> MEIALERIYGHRLALPQVGAALLFAQEAPPALLLVPEARLRRYRDLSAFGAKVYVNPGLEALEEKALFVLSYEEALSPFPEDPEAWRLLLEVGRAYPREALLSRLLKLGYARDEDYRVLGEVVELGEVRLEFFGDELERLVVRGEERRRHVLLPKPGKAEGFTSKKVLHFPGPVYLDTPALAPKALWPLLAGRPWVALGGGVELPPLELGARPLPPYRGSLKALEKDLARWLAEGKRVHLFVGHARTLEYLKRRLQAFSPLILDRFPGPKGRLALLPGDFEGGAEWGEWVLLTEALVFATGGVRARVRVGEGLSDPGALSPGDYLIHPEHGVGQYLGLETREVLGVKRDYLVLRYKGEGKLYLPVEQLPLLKRHPGTTDDPPELSSLGKNEWQRAKEKARKDVEELAGRLLVLQAKRKATPGRAFPPLPEWDPLVEKGFPYELTPDQKRALEEVLRDLESPHPMDRLVSGDVGFGKTEVALRAAHRVVGHGAQVAFLVPTTLLAEQHGKTFRERFQGLPVRVAVLSRFTPPKEEEAILKGLAEGTVDIVIGTHRLLQEDVRFRDLGLLIVDEEHRFGVAQKERIRELKAEVDTLYLSATPIPRTLYSALVGLKDLSSIQTPPPGRKPIKTFLAPFDPLLVREAILFELERGGKVFYVHDRVASIEARRRFLESLVPEARIGVVHGQMPESLIEETMLLFAEGAYDVLLATTIIEAGLDVPEANTILIERADRLGLATLYQLRGRVGRREEEAYAYLFHPPRLTEAAEKRLAAIADLSDLGSGHLLAERDMEIRGVGNLLGPEQHGHIRALSLEVYTELLEEAIRKLKGEVKEERRHVTLDLALSARLPAEYVGSLEARSRYYSRFAEAKSLAELSRLVRELKERYGPLPEEAENFVALARLRLVAERKGVVSITEGLTHLEVVFPRYPLDYDARGLKGLPYRVELTQYPPGFRLEKKGLRPRDYPEALMEVLYLF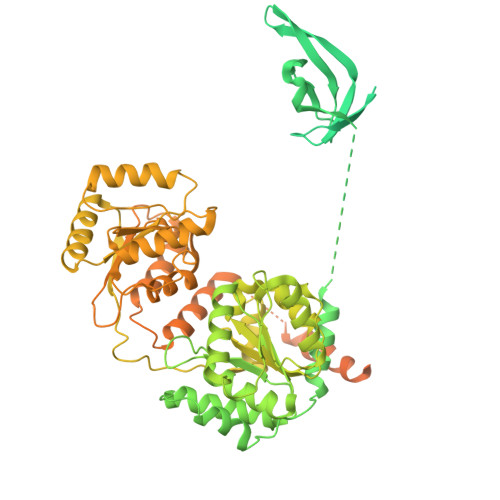ADL> ENGEGTTQPDYDNSTDYYNYEDFKCTCPAPHLNNTNGTVMKPIGCYYTCNVTRCTAPD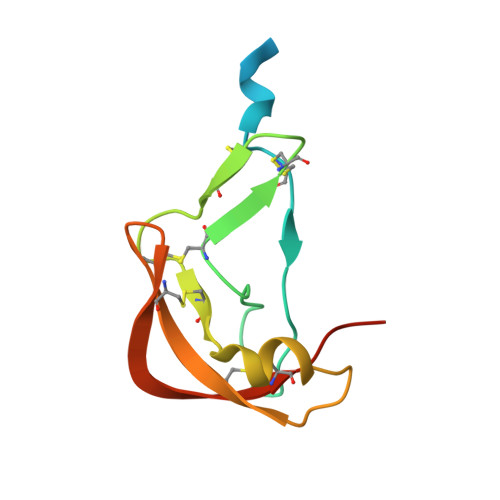TYPCYNLTEHQAKNLTTSPTTLCAVGNCDHGICVPNGTKELCFKAPNLEE> GNLTPEERDARTVFCMQLAARIRPRDLEEFFSTVGKVRDVRMISDRNSRRSKGIAYVEFVDVSSVPLAIGLTGQRVLGVPIIVQASQ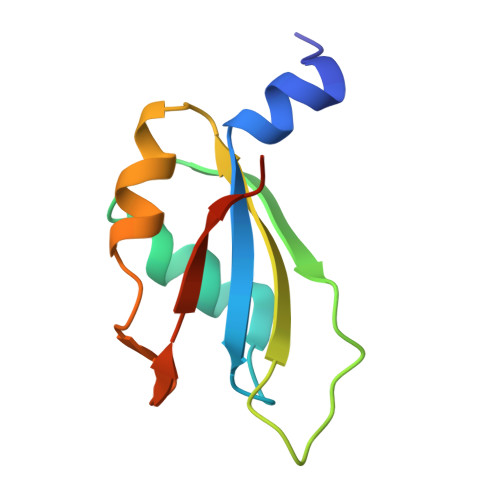AEKNR>MVLYFIGLGLYDERDITMKGLEIAKKCDYVFAEFYTSLMAGTTLGRIQKLIGKEIRVLSREDVELNFENIVLPLAKENDVAFLTPGDPLVATTHAELRIRAKRAGVESYVIHAPSIYSAVGITGLHIYKFGKSATVAYPEGNWFPTSYYDVIKENAERGLHTLLFLDIKAEKRMYMTANEAMELLLKVEDMKKGGVFTDDTLVVVLARAGSLNPTIRAGYVKDLIREDFGDPPHILIVPG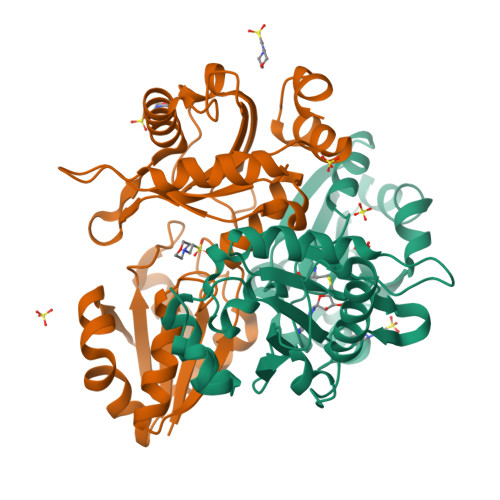KLHIVEAEYLVEIAGAPREILRVNV[2x]> MSLPSNPTPVIPANLDLGGINHSAVANRYRNLTKEAQQNLYQFAIIEVLSQIREERPDKNLDAYNALIGIDKVTTVDIYTYGATNMFFMPDARGSKTGILVNLNSPDKPYTNIQQPSDFNNINDESFRQNFTSWEKRDGTTYSGVDTALDGLQEGQGGWNLGYFNQKTPRTINISELSKILVERLDYHVSQENNDDQILSTLLLDVLPRSAKGAAREPLGVSASGIPFQLEFTFEGFTSPTDELRAIQSPFSHLAKYFDLLVASTNGSDLQDVEYSQEQAENIGAWIDSGTQLLMSASGIGAAVSVIQGAAGLTADAIEGKEIDPLDVISLSLAAIPGGKIVAKLSKVSKNLGQVVRGGISIAETGVDIVGSSRDLIEGFKKGNFTDIINGLVSVASSSASGRPGKSKIGNAIKKGNPDAPLPTRPTYRNHEGEVRPIPTAQTKSFFERVAIVRREGLSGRGAIGLDLTAAQKRGAELSGMGGTISKSNPNGNVSQVYINEAEGIEKNITYRKVPVPNEPGNFENRLQESFLDNNGQTKWRDFPYAGEEFDFRLQHKDDFNNIGDLGVGKQGIIAVNNPYSFVHHSHTFEQKGISNNHLTLESNAFLTYIEGKKTGDFENKYGNEMEWLVRKFKTKKNDFDLKDIPDNIHFRTDREKGDHSLTTYTLQDFITVVENAPTKMRKVKNDEFALNNIVESMRATAKNMGASPDTLFLDVASTNYMTQLMGQVLTNGRQELNLQGLSNAAQKLRNGASSSV

Combining experimental infection, cellular, and structural biology data, we demonstrated that nigritoxin is a potent toxin with lethal effect for crustaceans and insects. Nigritoxin is comprised of three domains, with the N-terminal domain being essential for cellular translocation and likely encoding specificity for Tetraconata, and the C-terminal domain being involved in cell death induction through apoptotic mechanisms. Typical signs of apoptosis were also observed in hemocytes of nigritoxin-injected shrimp and mimic cytopathological symptoms observed in animal infected by V. nigripulchritudo. This suggests that nigritoxin is a major virulence factor of V. nigripulchritudo and the hemocyte its primary target. Nigritoxin not only possesses a new protein fold but also seems to act by an original mechanism leading to apoptotic cell death.

The crystal structure of the nigritoxin was solved by the single anomalous diffusion (SAD) method, using a selenomethionine-labeled protein and refined at 2.1 Å resolution. The overall structural topology of nigritoxin is divided into three globular domains: a N-terminal (aa 17–268), a central (aa 276–460), and C-terminal domain (aa 495–753). A surface loop in the N-terminal domain contains a metal ion that was modeled as Mg2+, since this ion is present in the crystallization conditions. However, treatment of Sf9 cells with the chelating agent EDTA did not substantially alter the cytotoxic effect induced by nigritoxin, suggesting that the role of Mg2+ coordination is structural and not important for the activity. The C-terminal domain of nigritoxin contains two interesting and not yet described structural features: residues 512–544 form two large loops, each composed of two antiparallel strands that project out of the globular surface like “rabbit ears”. The bases of these protruding loops appear to be stabilized through a hydrophobic stacking of the side chain of Arg512 with the side chain of Trp540. The second feature is located on the concave side of the second, larger β-sheet, where four histidine residues and one arginine are concentrated in a groove with maximal distance of 10 Å creating a large and positively charged patch at the protein surface that has yet to have a defined biological function. Comparative analyses with Blast against PDB, DALI, Phyre2, or ProFunc revealed that neither the structure of full-length nigritoxin nor that of its individual subdomains resembles any known fold or protein structure, meaning that to date this protein structure is an “orphan”, making the identification of an active site difficult. On the other hand, deletion of the protruding loops eliminated toxicity, as did replacement with alanine of two histidine residues (His598 and His650) that are suspected of contributing to a functional “hotspot”.3-methoxy-~{N}-(1-methylpiperidin-1-ium-4-yl)-4-[[4-[(3-oxidanylidene-1,2-dihydroinden-4-yl)oxy]-5-(trifluoromethyl)pyrimidin-2-yl]amino]benzamide | C28 H29 F3 N5 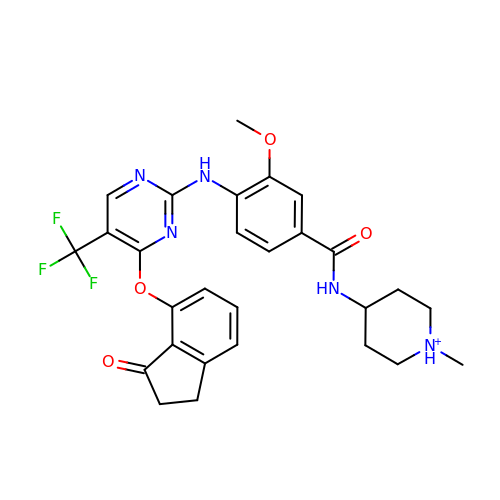O4 | QUSSZSMDFABHLI-UHFFFAOYSA-O Rab7A (Ras-related protein Rab-7a), a member of the Rab family of small GTPases, has been demonstrated to be a crucial regulator of mammalian autophagic and endosomal pathways. During mammalian autophagy, Rab7A can facilitate the maturation of autophagosomes and their fusion with lysosomes through its interactions with relevant regulatory proteins and binding partners. Particularly, the GDP (guanosine-5'-diphosphate) -bound inactive Rab7A is reported to be recruited to autophagosomes by its GEF (guanine nucleotide exchange factor) protein, the MON1/CCZ1/C18orf8 complex, which can specifically convert Rab7A to its GTP (guanosine-5'-triphosphate)-bound active state. However, due to the lack of complex structures, how the mammalian MON1 (monensin sensitivity 1)/CCZ1 (calcium caffeine zinc sensitivity 1)/C18orf8 (chromosome 18 open reading frame 8) complex specifically recognizes the GDP-bound inactive Rab7A and achieves its specific GEF activity for Rab7A remains unclear.

Then, based on previous structural studies of the fly Mon1/Ccz1/Bulli complex together with our relevant sequence alignment and Co-IP results, we used the truncated MON1A (235–652) fragment for assembling the MON1A/CCZ1/C18orf8 complex, and subsequently determined the Cryo-EM structure of the MON1A (235–652)/CCZ1 (1–482)/C18orf8 (1–657)/Rab7A (1–181) T22N complex to a 3.41 Å resolution, revealing a unique architecture of the MON1A/CCZ1/C18orf8 complex bound with one Rab7A (1–181) T22N. In the complex structure, both MON1A and CCZ1 are assembled in a triangular manner by three LD (Longin) domains, and directly interact with the C-terminal α-solenoid domain of C18orf8 forming the MON1A/CCZ1/C18orf8 complex. Meanwhile, Rab7A adopts a typical Rab GTPase fold, and packs against a solvent-exposed surface co-assembled by the two LD1 domains of MON1A and CCZ1 to form a triangular-like architecture. Further structural analyses of the binding interface of Rab7A (1–181) T22N with the MON1A/CCZ1/C18orf8 complex revealed that the specific association of Rab7A with the two LD1 domains of MON1A and CCZ1 is mainly mediated by both hydrophobic and hydrophilic interactions. Specifically, the hydrophobic side chain groups of Y37, I41 from the Switch I of Rab7A, and F45, W62 from the Interswitch as well as L73 from the Switch II of Rab7A occupy the hydrophobic groove formed by the V281, V283, A284, L285, and F288 residues from the MON1A LD1 domain and the L64, A67, and F71 residues from the CCZ1 LD1 domain. Furthermore, the side chains of K10, N22, T40, T58, Q60, Q67, E68, R79, and D82 together with the main chain carbonyl group of L8 from Rab7A interact with the A261, E273, G262, E260, N358, and D360 residues from MON1A LD1 and the E38, E66, and N56 residues from CCZ1 LD1, forming 10 specific hydrogen bonds. In parallel, the positively charged K31 and R69 from Rab7A couple with the negatively charged E238 from MON1A LD1 and E41 from CCZ1 LD1 to form two pairs of salt bridges, respectively.

> GTTEGDEEDATEAWRLHQKHVFVLSEAGKPVYSRYGSEEALSSTMGVMVALVSFLEADKNAIRSIHADGYKVVFVRRSPLVLVAVARTRQSAQELAQELLYIYYQILSLLTGAQLSHIFQQKQNYDLRRLLSGSERITDNLLQLMARDPSFLMGAARCLPLAAAVRDTVSASLQQARARSLVFSILLARNQLVALVRRKDQFLHPIDLHLLFNLISSSSSFREGEAWTPVCLPKFNAAGFFHAHISYLEPDTDLCLLLVSTDREDFFAVSDCRRRFQERLRKRGAHLALREALRTPYYSVAQVGIPDLRHFLYKSKSSGLFTSPEIEAPYTSEEEQERLLGLYQYLHSRAHNASRPLKTIYYTGPNENLLAWVTGAFELYMCYSPLGTKASAVSAIHKLMRWIRKEEDRLFILTPLTY;> MAAAAAGAGSGPWAAQEKQFPPALLSFFIYNPRFGPREGQEENKILFYHPNEVEKNEKIRNVGLCEAIVQFTRTFSPSKPAKSLHTQKNRQFFNEPEENFWMVMVVRNPIIEKQSKDGKPVIEYQEEELLDKVYSSVLRQCYSMYKLFNGTFLKAMEDGGVKLLKERLEKFFHRYLQTLHLQSCDLLDIFGGISFFPLDKMTYLKIQSFINRMEESLNIVKYTAFLYNDQLIWSGLEQDDMRILYKYLTTSLFPRHIEPELAGRDSPIRAEMPGNLQHYGRFLTGPLNLNDPDAKCRFPKIFVNTDDTYEELHLIVYKAMSAAVCFMIDASVHPTLDFCRRLDSIVGPQLTVLASDICEQFNINKRMSGSEKEPQFKFIYFNHMNLAEKSTVHMRKTPSVSLTSVHPDLMKILGDINSDFTRVDEDEEIIVKAMSDYWVVGKKSDRRELYVILNQKNANLIEVNEEVKKLCATQFNNIFFLD;> MGEEDYYLELCERPVQFEKANPVNCVFFDEANKQVFAVRSGGATGVVVKGPDDRNPISFRMDDKGEVKCIKFSLENKILAVQRTSKTVDFCNFIPDNSQLEYTQECKTKNANILGFCWTSSTEIVFITDQGIEFYQVLPEKRSLKLLKSHNLNVNWYMYCPESAVILLSTTVLENVLQPFHFRAGTMSKLPKFEIELPAAPKSTKPSLSERDIAMATIYGQLYVLFLRHHSRTSNSTGAEVVLYHLPREGACKKMHILKLNRTGKFALNVVDNLVVVHHQDTETSVIFDIKLRGEFDGSVTFHHPVLPARSIQPYQIPITGPAAVTSQSPVPCKLYSSSWIVFQPDIIISASQGYLWNLQVKLEPIVNLLPDKGRLMDFLLQRKECKMVILSVCSQMLSESDRASLPVIATVFDKLNHEYKKYLDAEQSYAMAVEAGQSRSSPLLKRPVRTQAVLDQSDVYTHVLSAFVEKKEMPHKFVIAVLMEYIRSLNQFQIAVQHYLHELVIKTLVQHNLFYMLHQFLQYHVLSDSKPLACLLLSLESFYPPAHQLSLDMLKRLSTANDEIVEVLLSKHQVLAALRFIRGIGGHDNISARKFLDAAKQTEDNMLFYTIFRFFEQRNQRLRGSPNFTPGEHCEEHVAFFKQIFGDQALMRPTTF;> MTSRKKVLLKVIILGDSGVGKNSLMNQYVNKKFSNQYKATIGADFLTKEVMVDDRLVTMQIWDTAGQERFQSLGVAFYRGADCCVLVFDVTAPNTFKTLDSWRDEFLIQASPRDPENFPFVVLGNKIDLENRQVATKRAQAWCYSKNNIPYFETSAKEAINVEQAFQTIARNALKQETEVELYNEFPEPIKLDKNDRAKASAESCSC>[3x]MPEGADPVAEVKTALAGFLKEVKGFQDDVKTRLQQQEERVTMLQTKTYAGRHALAAAATEEAPHQKAFAAYLRTGDDDGLRGLSLEGKALNSAVAAEGGYLVDPQTSETIRGVLRSTASLRQIASVVNVEATSFDVLVDKTDMGSGWASETAALSETATPQIDRITIPLHELAAMPKASQRLLDDSAFDIETWLANRIADKFARAEAAAFISGDGVDKPTGFLTKTKVANGAWAWGSLGYVATGAAGDFAAVNASDAVVDLVYALGAEYRANASFVMNSKTAGAVRKMKDADGRFLWADSLAAGEPARLMGYPVLIAEDMPDIAANAYAIAFGDFGNGYTIAERPDLRVLRDPFSAKPHVLFYASKRVGGDVSDFAAIKLLKFAAS

Gene transfer agents (GTAs) are DNA-containing phage-like particles produced by some species of bacteria and archaea. The genes encoding proteins that form Rhodobacter capsulatus GTA particles (RcGTA) are derived from phage DNA, which has been integrated into the bacterial genome. Here, we use cryo-electron microscopy (cryo-EM) to determine the structures of RcGTA before and after DNA ejection, and to visualize the interactions of RcGTA with R. capsulatus cells. Particles of RcGTA have heads with a diameter of 38-nm and 49-nm long tails.

One percent of the population of RcGTA are particles with isometric T = 3 icosahedral heads. The structure of the isometric RcGTA capsid with imposed icosahedral symmetry has been determined to a resolution of 4.0 Å. The existence of RcGTA particles with icosahedral heads provides evidence that the assembly of the oblate capsid is not based on intrinsic properties of the RcGTA major capsid protein but may be determined by scaffolding proteins. The quasi-equivalent structure of the T = 3 icosahedral capsid includes conformational differences in the major capsid proteins from one icosahedral asymmetric unit. In the major capsid proteins that form hexamers, the N-terminal arm, core helix from the peripheral domain, and extended loop lie in the same plane. By contrast, in the major capsid proteins which form pentamers, the structures are bent 18°, 8°, and 10° towards the center of the capsid. The planar quasi-hexamers in the icosahedral head are formed by capsid proteins in two alternating conformations, depending on whether they bind to pentamers or hexamers of capsid proteins. A particle of RcGTA with a T = 3 quasi-icosahedral head would not be capable of transferring its complete coding sequence; however, it would increase the chance that a combination of a few particles could transfer the whole coding sequence in segments to one recipient. If the RcGTA particles with icosahedral heads acquired the ability to preferentially package their coding sequences, they could become self-propagating and revert to a bacteriophage-like lifestyle.> ARHVLLQAEFYQRSEGPDKAWAQFGFHFDADELFHVELDAAQTVWRLPEFGRFASFEAQGALQNMAVGKQNLEVMISNSNRSQQDFVTPELALFPAEAVSLEEPNVLICYADKFWPPVATMEWRRNGAVVSEGV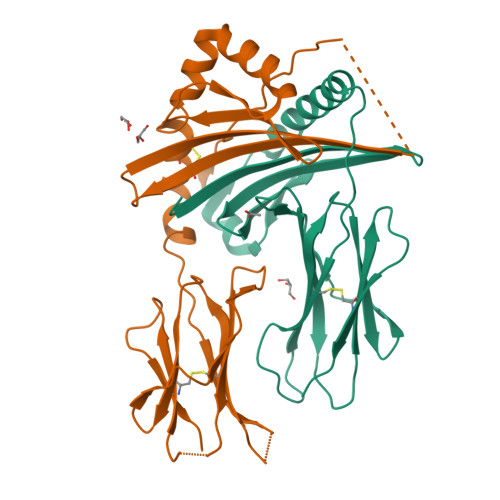YDSVYYGRPDLLFRKFSYLPFVPQRGDVYSCAVRHWGAEGPVQRMWEPE;> ADRPQIESLSLNGVPNIFLSTKAGGGGSGGGGSGGGGSSAFFFCGAIFECHYLNGTERVRYLQRYIYNRQQLVHFDSDVGKFVADTPLGEPQAEYWNSNAELLENIMNIADGSCRHNYGILESFTVQRSVEPKVRVSALQSGSLPETDRLACYVTGFYPPEIEVKWFLNGREETERVVSTDVMQNGDWTYQVLVVLETVPRRGDSYVCRVEHASLRQPISQAWE> GAMEDITSGLKQLDSTYQETNQQVLKNLDEIFSTTSPSANNEMGEEDALNIATAAIALRGDLALLKANFEANELFFISEDVIFKTYMSSPELLLTYMKINPLDQNTAEQQCGISDKVLVLYCEGKLKIEATAQNIRERLETSLKAYQSNIGGTASLITASQTLVESLKNKNFIKGIRK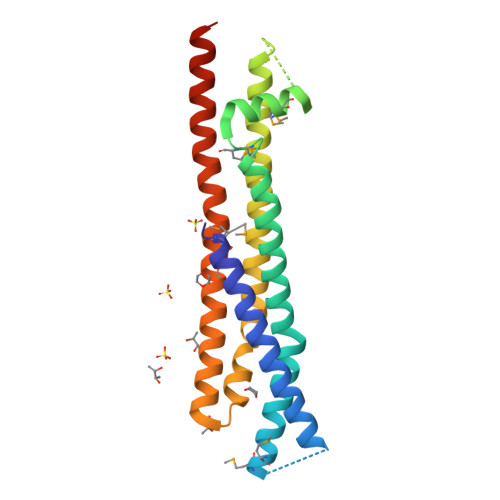LMLAHNKVFLNYLEELDALERSLEQSKRQYLQERQSSKIIVK Molybdenum- or tungsten-dependent formate dehydrogenases have emerged as significant catalysts for the chemical reduction of CO2 to formate, with biotechnological applications envisaged in climate-change mitigation. In the particular case of the tungsten FdhAB from Desulfovibrio vulgaris (DvFdhAB), a selenocysteine coordinates the tungsten ion and the enzyme displays a simple heterodimeric structure: a catalytic α subunit (harbouring the tungsten active site and one [4Fe–4S] centre) and a β subunit (with three [4Fe–4S] clusters) involved in electron transfer to/from electron acceptors/donors. In the active site, the Mo/W atom coordinates two dithiolenes from two molybdopterin guanine dinucleotides (MGDs), one terminal sulfido ligand (—SH/=S) and a (seleno)cysteine residue from the polypeptide chain in a distorted trigonal prismatic geometry. The allosteric mechanism involves large conformational changes, namely of the side chain of Met405, a residue located near the active site that is fully conserved in the subclass of Fdhs that contain the recently reported allo­steric redox switch for protection against oxygen-induced damage.

In this work, the M405S variant was engineered, which allowed the active-site geometry in the absence of methionine Sδ interactions with the metal site to be revealed and the role of Met405 in catalysis to be probed. The mutation of Met405 to serine (or alanine) led the Gln409 side chain to occupy the space left vacant by the absence of the Met405 side chain, resulting in a backbone rearrangement that pulls Thr408 4.3 Å away from its original position and causes it to interact with the protein backbone near U192. Additionally, the catalytically essential residue His193 displays a new conformation that is closer to that in the oxidized WT enzyme, but is intermediate between the oxidized and reduced states. Therefore, this new conformation, which is associated with increased backbone flexibility, is likely to interfere with the catalytic role of His193, possibly accounting for some of the loss of activity of the M405S variant. Met405 was previously assigned to play a key structural role, but only in the present M405S variant could we confirm the significant rearrangement of the Ile191–Thr196 helical region (particularly the mechanistically relevant residues U192 and His193) and the consequent distortion of the metal coordination geometry.

> MTVTRRHFLKLSAGAAVAGAFTGLGLSLAPTVARAELQKLQWAKQTTSICCYCAVGCGLIVHTAKDGQGRAVNVEGDPDHPINEGSLCPKGASIFQLGENDQRGTQPLYRAPFSDTWKPVTWDFALTEIAKRIKKTRDASFTEKNAAGDLVNRTEAIASFGSAAMDNEECWAYGNILRSLGLVYIEHQARIUHSPTVPALAESFGRGAMTNHWNDLANSDCILIMGSNAAENHPIAFKWVLRAKDKGATLIHVDPRFTRTSARCDVYAPIRSGADIPFLGGLIKYILDNKLYFTDYVREYTNASLIVGEKFSFKDGLFSGYDAANKKYDKSMWAFELDANGVPKRDPALKHPRCVINLLKKHYERYNLDKVAAITGTSKEQLQQVYKAYAATGKPDKAGTIMYASGWTQHSVGVQNIRAMAMIQLLLGNIGVAGGGVNALRGESNVQGSTDQGLLAHIWPGYNPVPNSKAATLELYNAATPQSKDPMSVNWWQNRPKYVASYLKALYPDEEPAAAYDYLPRIDAGRKLTDYFWLNIFEKMDKGEFKGLFAWGMNPACGGANANKNRKAMGKLEWLVNVNLFENETSSFWKGPGMNPAEIGTEVFFLPCCVSIEKEGSVANSGRWMQWRYRGPKPYAETKPDGDIMLDMFKKVRELYAKEGGAYPAPIAKLNIADWEEHNEFSPTKVAKLMNGYFLKDTEVGGKQFKKGQQVPSFAFLTADGSTCSGNWLHAGSFTDAGNLMARRDKTQTPEQARIGLFPNWSFCWPVNRRILYNRASVDKTGKPWNPAKAVIEWKDGKWVGDVVDGGGDPGTKHPFIMQTHGFGALYGPGREEGPFPEHYEPLECPVSKNPFSKQLHNPVAFQIEGEKKAVCDPRYPFIGTTYRVTEHWQTGLMTRRCAWLVEAEPQIFCEISKELAKLRGIGNGDTVKVSSLRGALEAVAIVTERIRPFKIEGVDVHMVGLPWHYGWMVPKNGGDTANLLTPSAGDPNTGIPETKAFMVDVRKVWSHPQFEK;> MGKMFFVDLSRCTACRGCQIACKQWKNLPAEETRNTGSHQNPPDLSYVTLKTVRFTEKSRKGPGIDWLFFPEQCRHCVEPPCKGQADVDLEGAVVKDETTGAVLFTELTAKVDGESVRSACPYDIPRIDPVTKRLSKCDMCNDRVQNGLLPACVKTCPTGTMNFGDEQEMLALAEKRLAEVKKTYPGAVLGDPNDVRVVYLFTRDPKDFYEHAVA>SDDLSFKFKNFSQNGKDLSFQGNASVIETGVLQLNKVGNNLPDETGGIARYIAPIHIWNCNTGELASFITSFSFFMETSANPKAATDGLTFFLAPPDSPLRRAGGYFGLFNDTKCDSSYQTVAVEFDTIGSPVNFWDPGFPHIGIDVNCVKSINAERWNKRYGLNNVANVEIIYEASSKTLTASLTYPSDQTSISVTSIVDLKEILPEWVSVGFSGSTYIGRQATHEVLNWYF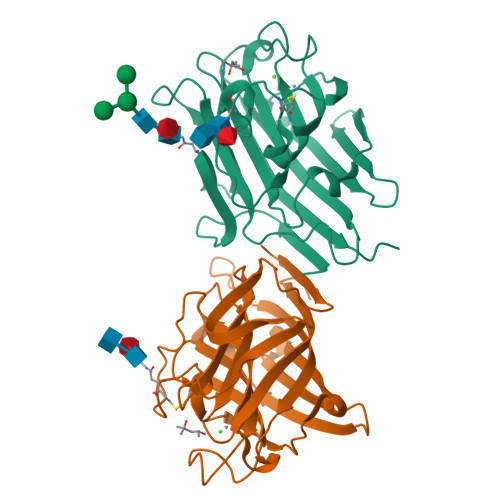TSTFINTNS[2x]> VMLTRQQKELIVKEMSEIFKKTSLILFADFLGFTVADLTELRSRLREKYGDGARFRVVKNTLLNLALKNAEYEGYEEFLKGPTAVLYVTEGDPVEAVKIIYNFYKDKKADLSRLKGGFLEGKKFTAEEVENIAKLPSKEELYAMLVGRVKAPITGL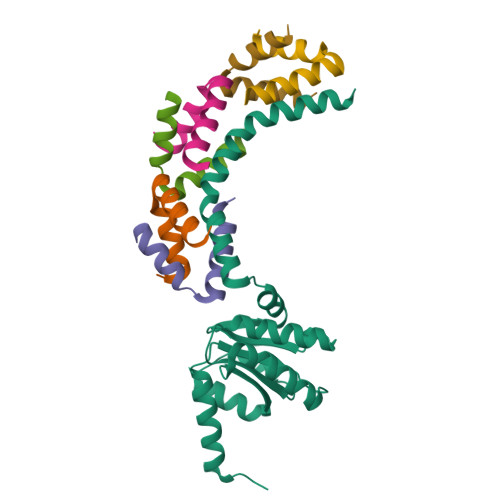VFALSGILRNLVYVLNAIKEKKSE;>MTIDEIIEAIEKLTVSELAELVKKLEDKFG[6x]> MSAKDERAREILRGFKLNWMNLRDAETGKILWQGTEDLSVPGVEHEARVPKKILKCKAVSRELNFSSTEQMEKFRLEQKVYFKGQCLEEWFFEFGFVIPNSTNTWQSLIEAAPESQMMPASVLTGNVIIETKFFDDDLLVSTSRVRLFYV

RAS is a major anticancer drug target which requires membrane localization to activate downstream signal transduction. Phosphodiesterase 6δ (PDE6D) has a beta-sandwich immunoglobulin fold which contains a hydrophobic pocket capable of binding to the farnesyl group. PDE6D binds to and sequesters the lipid of cytoplasmic RAS and has been proposed to deliver GTPase to recycling endosomes, which is followed by release mediated by the small G-protein Arf-like 2 (ARL2), allowing RAS to be trafficked back to the plasma membrane. The resultant lipid modification increases the affinity of RAS proteins toward membranes, where it is required for signal transduction. Here, we present a novel strategy for targeting RAS by stabilizing its interaction with the prenyl-binding protein PDE6D and disrupting its localization.

Within their HVR sequences, both HRAS and NRAS contain a cysteine residue in the −5 position relative to the modified C-terminal cysteine. We were successfully able to cocrystallize PDE6D with C-terminally modified peptides of both HRAS and NRAS. In the crystal structure of the NRAS HVR bound to PDE6D, the electron density for only the farnesyl can be interpreted. This is most likely due to the flexibility of the peptide, whose composition, including a proline in the −1 and glycine in the −3 position relative to the lipidated cysteine, could provide unique conformational restraints compared to the other RAS isoforms. As NRAS has a cysteine in the −5 position, analogously to HRAS, it is likely that the cysteine would be in a similar conformation. We therefore hypothesized that these cysteine residues could be targeted to irreversibly attach an inhibitor to both HRAS and NRAS, generating RAS isoform-specific PDE6D stabilizers.> MNDETLTVYRGATDNKGNPNKQVHGTV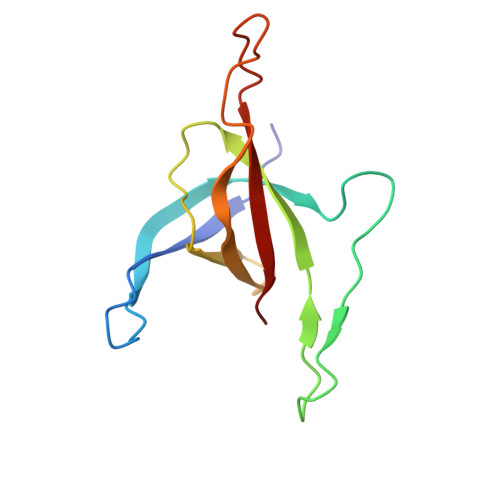KGVFAWGPGTSTNKFGRDRNFKGESSSLTAELYVKRGADLKARDRIRRANGEEYSVVGHAAWDQGHPFDGFDFGYMVFQVEAVN>SMAEIRISWWGGNQRHEATLAAINAFQKANPTITVKAEYAGWDGYLSRLSTQIAGGQEPDVMRIDWNWLPQFSRNGDGFYDLNKQKDILGLGDFPPNALKTADVKGKLQGLPISMTSRSMIYNKTTWDNAGVAYPKTWDELFAAGPVFKQKLGDSYYPLGVAQGASDVLDILTLGRSYMAQKYGIDMIDEKKQSIAYSRDQVRELFGFYKKLVDSHVIPDQRYFSSFGRTNVYEIRPWINGELAGMYLWDSAIYTYSSNMPKDAVLETGPFITIPGAKDSGLTSKPSSLFAISKNSKHPKEAAMLMNFMLSNPEGVKALGLQNGMPANPKAQKLLEDIGVINPGNLLANAYRAAAAQP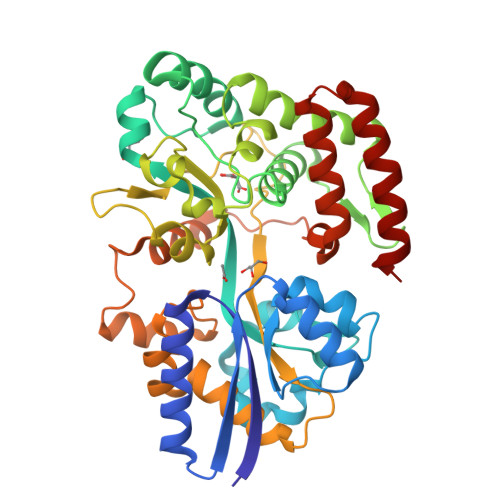ESKVAVSPFMENQELVQLWTTSLQKLDYGNGEVNKVADDFLSGANRILKRAIR[2x]(1S)-1-[3-(cyclohexylmethoxy)phenyl]propane-1,3-diol 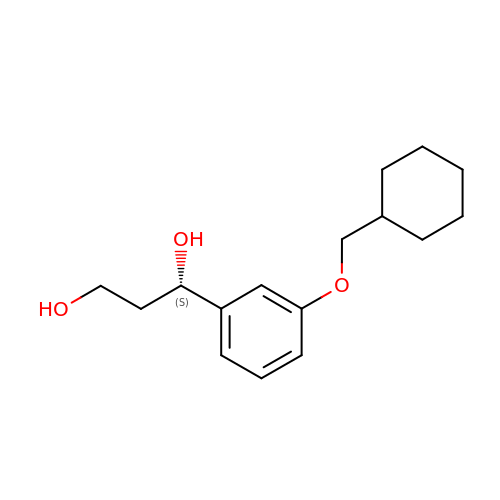| C16 H24 O3 | JEPZJYPEDPLQFU-INIZCTEOSA-N>ASMTGGQQMGRGSEFMGQSHTHDHHHDGYQAPPEDIALRVKALESLLIEKGLVDPAAMDLVVQTYEHKVGPRNGAKVVAKAWVDPAYKARLLADGTAGIAELGFSGVQGEDMVILENTPAVHNVFVCTLCSCYPWPTLGLPPAWYKAAPYRSRMVSDPRGVLAEFGLVIPANKEIRVWDTTAELRYMVLPERPAGTEAYSEEQLAELVTRDSMIGTGLPTQPTPSH[4x];>[4x]MNGIHDTGGAHGYGPVYREPNEPVFRYDWEKTVMSLLPALLANGNFNLDEFRHSIE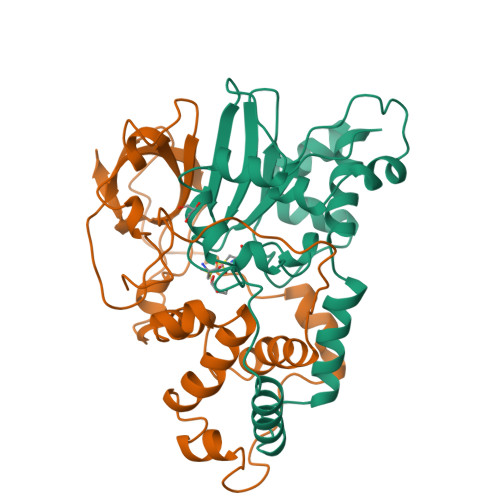RMGPAHYLEGTYYEHWLHVFENLLVEKGVLTATEVATGKAASGKTATPVLTPAIVDGLLSTGASAAREEGARARFAVGDKVRVLNKNPVGHTRMPRYTRGKVGTVVIDHGVFVTPDTAAHGKGEHPQHVYTVSFTSVELWGQDASSPKDTIRVDLWDDYLEPA>[3x]GPLSSPADSYNEGVKLQPQEISPPPTANLDRSNDKVYENVTGLVKAVIEMSSKIQPAPPEEYVPMVKEVGLALRTLLATVDETIP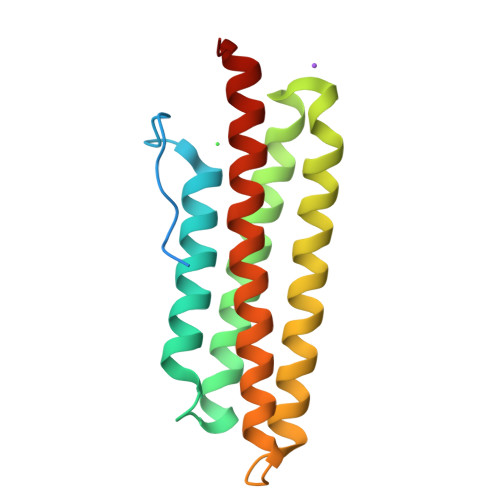LLPASTHREIEMAQKLLNSDLGELINKMKLAQQYVMTSLQQEYKKQMLTAAHALAVDAKNLLDVIDQARLKMLGQTRPH> MQKIGILGAMREEITPILELFGVDFEEIPLGGNVFHKGVYHNKEIIVAYSKIGKVHSTLTTTSMILAFGVQKVLFSGVAGSLVKDLKINDLLVATQ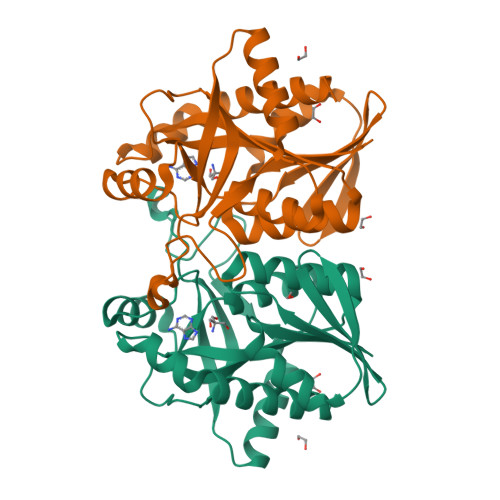LVQHDVDLSAFDHPLGFIPESAIFIETSGSLNALAKKIANEQHIALKEGVIASGDQFVHSKERKEFLVSEFKASAVEMEGASVAFVCQKFGVPCCVLRSISDNADEKAGMSFDEFLEKSAHTSAKFLKSMVDEL> GDATTARGDSVEFDFFAAPQAYRRVAAEHRADGAFHSSRGDSFWVLSTYEGICAAFRDEDTFSVSRVSAADGAEDERWIPLTIQGRTHNEWRRRLAAWFTPQRARDLTPAIRANARRRISAFVDRGEVSFSDEFARPYVLENLMLAVGWPLADLDHLLAINVAMIRSREAPDPRQAFNAETAFPALQEYVRRHVARRRTEPVEGDLTSATFDWEIDGT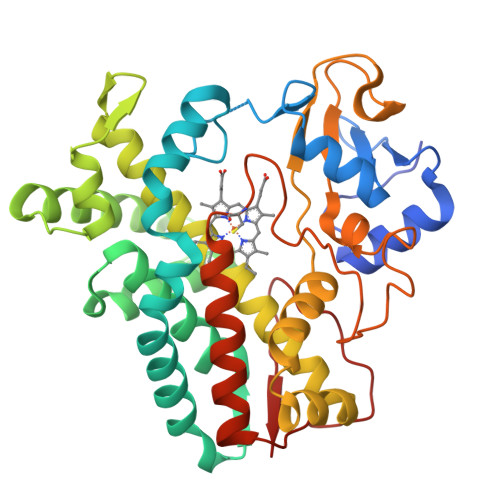PVSDADRESLLTVLFLAGVDSTVNHMANGIQHLAHHPGDRHRFLRDPEVRPAAVEEFLRVNSCMYPGRLATREGAGGVASQGDTVLLPLALANYDPAVFPEPERVDFDREQNPHIAFGTGHHQCLGAAYARAQILTAWEEWHELIPDYRLPDPTVEPPFLRNVYDLRIVW>[8x]KKLAEYKCNTNTAIELKLVRFPEDLENDIRTFFPEYTHQLFGDDETAFGYKGLKILLYYIAGSLSTMFRVEYASKVDENFDCVEADDVEGKIRQIIPPGFCTNTNDFLSLLEKEVDFKPFGTLLHTYSVLSPTGGENFTFQIYKADMTCRGFREYHERLQTFLMWFIETASFIDVDDERWHYFLVFEKYNKDG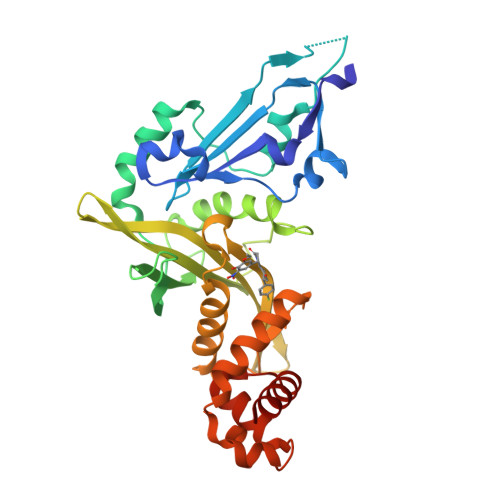ATLFATVGYMTVYNYYVYPDKTRPRVSQMLILTPFQGQGHGAQLLETVHRYYTEFPTVLDITAEDPSKSYVKLRDFVLVKLCQDLPCFSREKLMQGFNEDMAIEAQQKFKINKQHARRVYEILRLLVTD> MQAQYCSVNKDIFEVEENTNVTEPLVDIHVPEGQEVTLGALSTPFAFRIQGNQLFLNVTPDYEEKSLLEAQLLCQSGGTLVTQLRVFVSVLDVNDNAPEFPFKTKEIRVEEDTKVNSTVIPETQLQAEDRDKDDILFYTLQEMTAGASDYFSLVSVNRPALRLDRPLDFYERPNMTFWLLVRDTPGENVE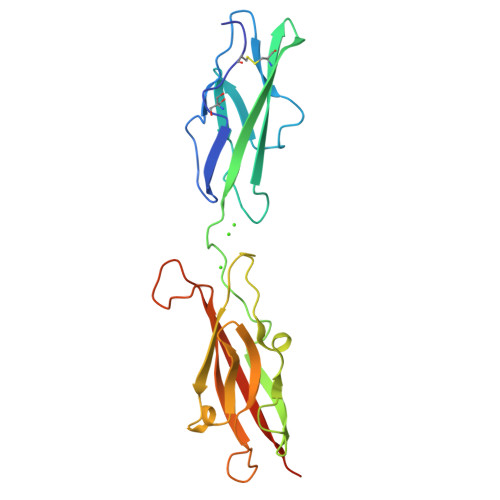PSHTATATLVLNVVPADLEHHHHHH decyl 4-O-alpha-D-glucopyranosyl-1-thio-beta-D-glucopyranoside | C22 H42 O10 S | 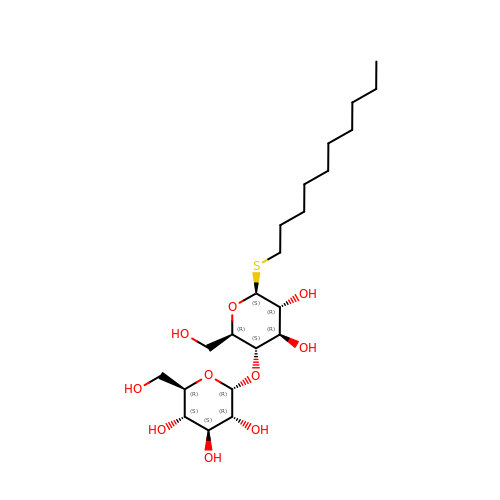YZNNXXWNKQOETJ-HYLFJBCQSA-N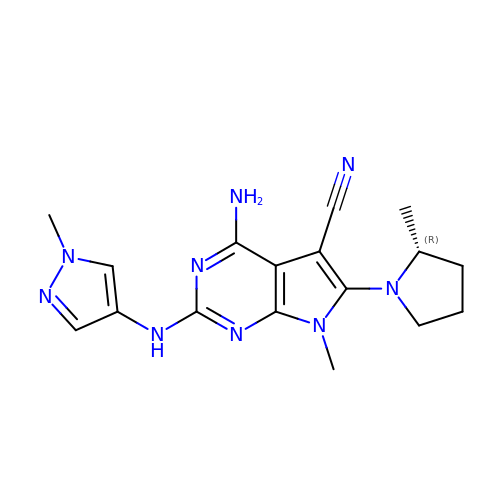4-amino-7-methyl-2-[(1-methyl-1H-pyrazol-4-yl)amino]-6-[(2R)-2-methylpyrrolidin-1-yl]-7H-pyrrolo[2,3-d]pyrimidine-5-carbonitrile | C17 H21 N9 | QQIQPTYOVZSTDB-SNVBAGLBSA-N> XSLSDKDKAAVKLLWSKISKSSDAIGNDALSRMIVVYPQTKTYFAHWPDLSPGSPHVKAHGKTVMGGIALAVSKIDDLRAGLLDLSEQHAYKLRVDPANFKILSHCILVVISMMFPKEFTPEAHVSLDKFLSGVSLALSERYR;> VEWTDQERATISSIFGSLDYDDIGPKALSRCLIVYPWTQRHFGSFGNLYNAEAIIGNQKVAAHGIKVLHGLDRAVKNMDNIKEIYAELSILHSEKLHVDPDNFKLLADCLTIVVAAKMGSGFNPGTQATFQKFLAVVVSALGKQ

The superfamily of globins includes proteins that are ubiquitous in a variety of different living organisms, from bacteria to higher eukaryotes, where they perform key functions essentially related to their ability to bind gaseous ligands. The globin fold is made of six to eight helices that constitute the matrix where the heme group, which is deputed to the ligand binding, is anchored. In this scenario, we have undertaken the biochemical and biophysical characterization of the Hb isolated from the sub-Antarctic notothenioid fish Eleginops maclovinus (Hb1Em) that lives in the Beagle Channel surrounding the Tierra del Fuego (Argentina) by experiencing temperature ranges from 4 °C to 10 °C32. Particularly, Hb1Em exhibits the Root effect (drastic drop of oxygen cooperativity at low pH) that is physiologically necessary to secrete O2 against high O2 pressures into the swimbladder or the retina, following local acidification of the blood in a counter-current capillary system.

Here, we report the structure of a second carbomonoxy form that presents several structural properties that are unique for globin structures. In the α chain a striking rearrangement of the heme pocket is observed: the side chain of the distal His59α, which assumes a canonical location in Hb1EmCO_ortho, is far from the heme group. Indeed, the distance between the Nε2 atom of His59α and the oxygen atom of the CO ligand, which are at hydrogen-bonding distance in canonical carbonmonoxy Hbs, is 10.3 Å in Hb1EmCO_hexa. This unique location of His59α is favored by the helix E distortion and stabilized by the formation of several stabilizing interactions. The most evident one is the strong electrostatic interaction established by His59α and Asp48α side chains. The displacement of His59α produces a rearrangement of the distal side of the heme pocket characterized by a movement of the side chains of the hydrophobic residues Phe43α, Trp46α, and Leu29α that, compared to Hb1EmCO_ortho, become closer to the CO molecule. Interestingly, the rearrangement of the overall architecture of the distal side observed in Hb1EmCO_hexa is unique among vertebrate globins. The inspection of the RMSD values shows that the quaternary structure of Hb1EmCO_hexa is quite different from that exhibited by Hb1EmCO_ortho (RMSD of 2.16 Å). The evidence in Hb1EmCO_hexa of a stable carbomonoxy form in a T quaternary state is in perfect agreement with a biphasic CO-dissociation kinetic and with the stopped-flow kinetic curves previously observed for the Hb of E. maclovinus.>[3x]GPGSGPRPAQLTWSQLPEVLESGVLDTLSTEERKRQEAIFEILTSEFSYLHSLSILVTEFLQSRELRATMTQTEHHHLFSNILDVMSASQKFFEALEQRHKAQVCVEDISDILEDHAQHHFHPYIAYCSNEVYQQRTLQKLSNSNAAFRDVLKEIEKRPACGGLPMISFLILPMQRVTRLPLLTDTLCLKTQGHPERYKAASQALKAISKLVKQCNEGAHKMERTEQIYTLNMQLDF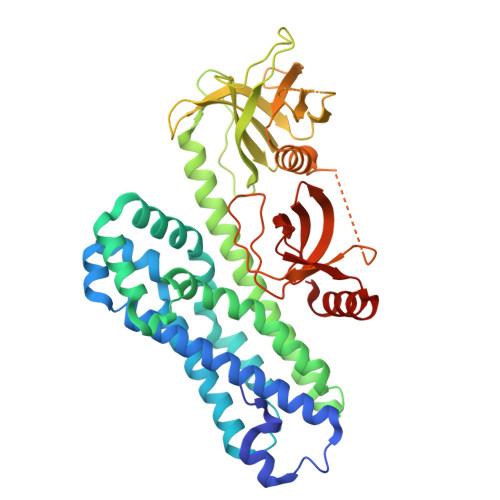GKVKSLPLISASRWLLKRGELFLLEESSIFRKIASRPTCYLFLFNDVLVVTKKKSEESYLVQDYAQLDHVQVRKLEPSEPLLPGGSSRSSSVPYPFQVNLLHNSEGRQEQILLSSDSASDRARWITALTYKERQWQGITNKGELPQVEVTKAYFAKQADEITLQQADIVLVLQEEDGWLHGERLLDGETGWFPESFAHSITSRVAVEGNVRRMERLRVETDV>MAMQAAKRANIRLPPEVNRILYIRNLPYKITAEEMYDIFGKYGP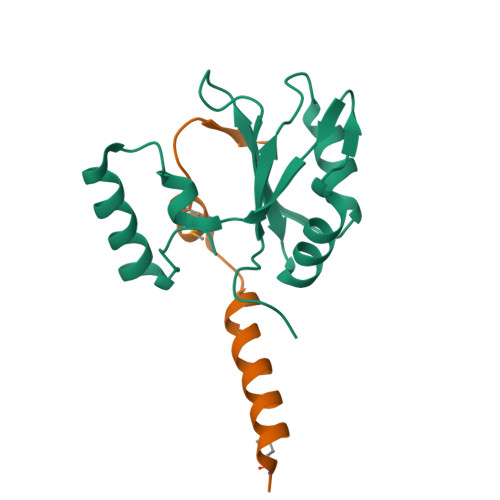IRQIRVGNTPETRGTAYVVYEDIFDAKNACDHLSGFNVCNRYLVVLYYNANRAFQKMDTKKKEEQLKLLKEKYGINTDPPK[2x];>[2x]GHIMSMTPEQLQAWRWEREIDERNRPLSDEELDAMFPEGYKVL>[12x]MTGNDVQGAEKADAIGMVLGTEDVTPTVFWFAVSHGASVGLDDLVVVETRKPDGTPVRFYGLVDNVRKRHEGVTFESDVEDVVAGLLPASVSYAARVLVTRVDPENFIPPQPGDHVRHAAGRELAMALSADKMEEAAFPGGLLADGQPLPLNFRFINGESGGHINISGISGVATKTSYALFLLHSIFRSGVMDRTAQGSGGRQSGTAGGRALIFNVKGEDLLFLDKPNARMVEKEDKVVRAKGLSADRYALLGLPAEPFRDVQLLAPPRAGAAGTAIVPQTDQRSEGVTPFVFTIREFCARRMLPYVFSDASASLNLGFVIGNIEEKLFRLAAAQTGKGTGLIVHDWQFEDSETPPENLDFSELGGVNLQTFEQLISYLEYKLLEEREGEGDPKWVLKQSPGTLRAFTRRLRGVQKYLSPLIRGDLTPEQAEG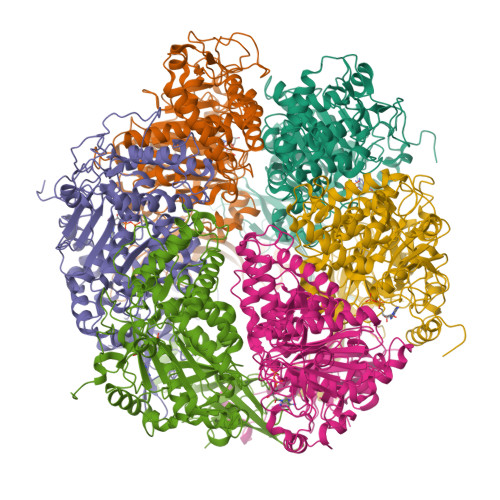YRPDPLRRGIQLTVVDIHALSAHAQMFVVGVLLREVFEYKERVGRQDTVFVVLDELNKYAPREGDSPIKDVLLDIAERGRSLGIILIGAQQTASEVERRIVSNAAIRVVGRLDLAEAERPEYRFLPQSFRGRAGILQPGTMLVSQPDVPNPVLVNYPFPAWATRRDEVDDLGGKAAAEVGAGLLR> MVFDVWKSLKKGEVHPVYCLYGKETYLLQE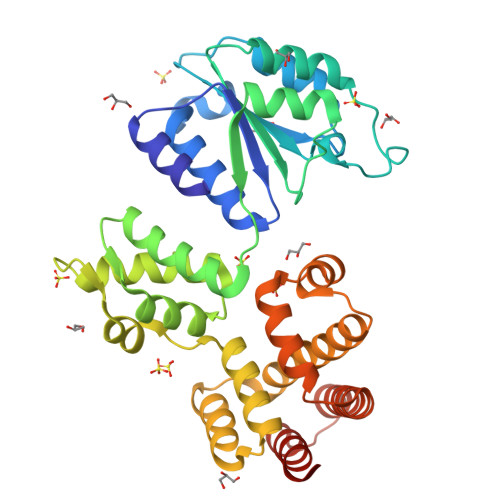TVSRIRQTVVDQETKDFNLSVFDLEEDPLDQAIADAETFPFMGERRLVIVKNPYFLTGEKKKEKIEHNVSALESYIQSPAPYTVFVLLAPYEKLDERKKLTKALKKHAFMMEAKELNAKETTDFTVNLAKTEQKTIGTEAAEHLVLLVNGHLSSIFQEIQKLCTFIGDREEITLDDVKMLVARSLEQNIFELINKIVNRKRTESLQIFYDLLKQNEEPIKIMALISNQFRLILQTKYFAEQGYGQKQIASNLKVHPFRVKLAMDQARLFSEEELRLIIEQLAVMDYEMKTGKKDKQLLLELFLLQLLKRNEKNDPHY>[2x]CGCIA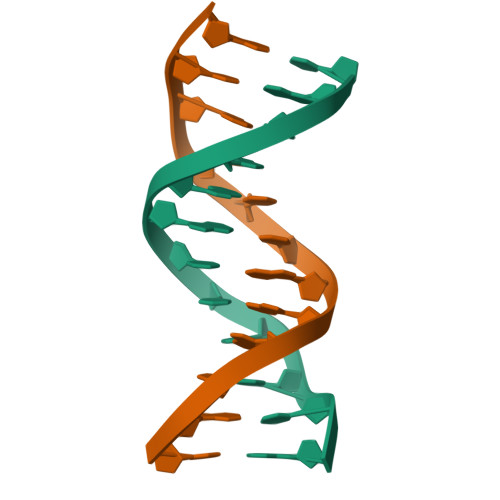ATTCGCG>[2x]MHHHHHHSAGENLYFQGKEWQENKSWNAHFT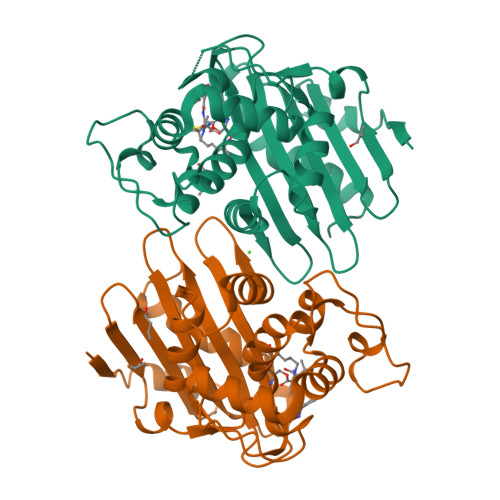EHKSQGVVVLWNENKQQGFTNNLKRANQAFLPASTFKIPNSLIALDLGVVKDEHQVFKWDGQTRDIATWNRDHNLITAMKYSVVPVYQEFARQIGEARMSKMLHAFDYGNEDISGNVDSFWLDGGIRISATEQISFLRKLYHNKLHVSERSQRIVKQAMLTEANGDYIIRAKTGYSTRIEPKIGWWVGWVELDDNVWFFAMNMDMPTSDGLGLRQAITKEVLKQEKIIP>[4x]SFETRFEKMDNLLRDPKSEVNSDCLLDGLDALVYDLDFPALRKNKNIDNFLSRYKDTINKIRDLRMKAEDYEVVKVIGRGAFGEVQLVRHKSTRKVYAMKLLSKF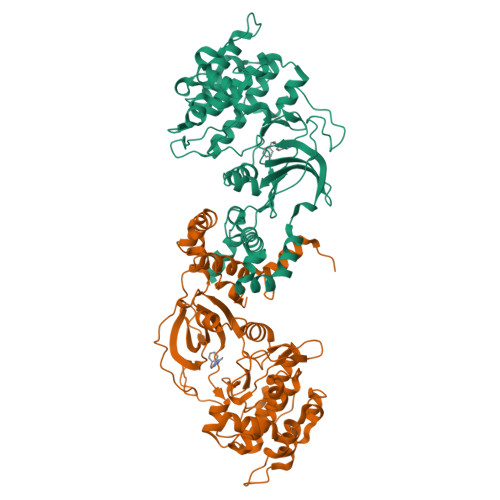EMIKRSDSAFFWEERDIMAFANSPWVVQLFYAFQDDRYLYMVMEYMPGGDLVNLMSNYDVPEKWARFYTAEVVLALDAIHSMGFIHRDVKPDNMLLDKSGHLKLADFGTCMKMNKEGMVRCDTAVGTPDYISPEVLKSQGGDGYYGRECDWWSVGVFLYEMLVGDTPFYADSLVGTYSKIMNHKNSLTFPDDNDISKEAKNLICAFLTDREVRLGRNGVEEIKRHLFFKNDQWAWETLRDTVAPVVPDLSSDIDTSNFDDLEEDKGEEETFPIPKAFVGNQLPFVGFTYYSNRRYLSSANPNDNR Lytic polysaccharide monooxygenases [LPMOs, reviewed in Tandrup et al., Vu & Ngo, Wang et al. and Eijsink et al.] were discovered just over 10 years ago and are metalloenzymes containing a type II Cu centre. A Cu2+ ion is coordinated by two histidines in a motif known as the histidine brace (His-brace), where the N-terminal His is often Nɛ2-methyl­ated in LPMOs of fungal origin and coordinates Cu using both the N-terminal nitro­gen and the Nδ1 atom. LPMOs cleave the glycosidic bond, producing both oxidized (C1 and/or C4) and non-oxidized chain ends. Here we have monitored the Cu-site geometry in two AA9 LPMOs, one from Lentinus similis (LsAA9_A) and one from Thermoascus auranti­acus (TaAA9_A), as the active-site Cu is photoreduced in the X-ray beam.

Additionally, we have solved six structures of the C1/C4-oxidizing AA9 from Thermoascus auranti­acus (TaAA9_A, where oligosaccharides bound in the structure have so far not been obtained) to identify similarities between AA9s as the central Cu ion is reduced. TaAA9_A has been used previously in describing the LPMO active site in theoretical studies and the structures here could therefore present an improvement for further calculations. Crystal contacts most likely prevent binding at negative subsites, assuming the oligosaccharide binds in a similar manner to previous oligosaccharide-binding structures with LsAA9_A and an AA9 from Collariella virescens (CvAA9_A), and it has not been possible so far to obtain an oligosaccharide bound in the structure of this protein, which also has no reported activity on oligosaccharides. In a previous EXAFS study, it was indicated that the Cu2+ structure of TaAA9_A could be well represented by four N/O ligands at an average distance from Cu of 1.98 Å, whereby one of the close ligands was lost on photoreduction, leaving the Cu atom in a T-shaped coordination. The equatorial ligand distances in the lowest-dose TaAA9_A structure presented have an average of 2.1 Å, which is within the agreement level that can be expected given an estimated coordinate error of 0.207 Å for this structure; however, in the crystal structure, an axial water is additionally very close at a distance from Cu of 2.0 Å and is significantly closer than in the LsAA9_A substrate-free structures above. The equatorial water mol­ecule sits at 2.2 Å from the Cu atom in the lowest-dose structure and reaches the longest distance of 2.6 Å at an inter­mediate dose (1.13 × 106 Gy).

> HGFVQNIVIDGKNYGGYLVNQYPYMSNPPEVIAWSTTATDLGFVDGTGYQTPDIICHRGAKPGALTAPVSPGGTVELQWTPWPDSHHGPVINYLAPCNGDCSTVDKTQLEFFKIAESGLINDDNPPGIWASDNLIAANNSWTVTIPTTIAPGNYVLRHEIIALHSAQNQDGAQNYPQCINLQVTGGGSDNPAGTLGTALYHDTDPGILINIYQKLSSYIIPGPPLYTG>[6x]AHMGNTKLANPAPLGLMGFGMTTILLNLHNVGYFALDGIILAMGIFYGGIAQIFAGLLEYKKGNTFGLTAFTSYGSFWLTLVAILLMPKLGLTDAPNA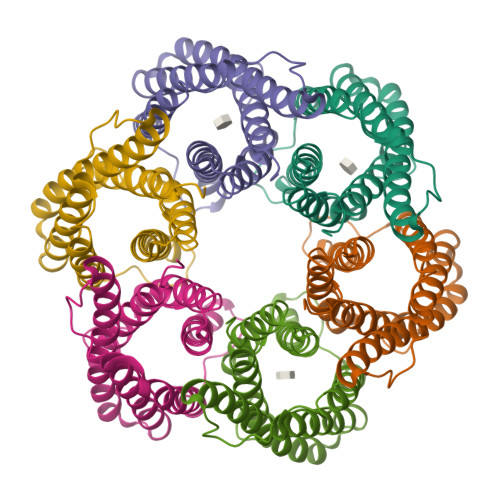QFLGVYLGLWGVFTLFMFFGTLKGARVLQFVFFSLTVLFALLAIGNIAGNAAIIHFAGWIGLICGASAIYLAMGEVLNEQFGRTVLPIGESH> MNNWQHFFNNPVDLSEHLKKPYFRFDNRDKEITAISFDEKANLIWSGDSYGCISSYDPTFQLYTRYRGHIGGNSVKDILSHRDGILSISEDSLHFANRRGVTKLNLTSIDIAAFSELNTMCYSPHSLKNNIYCGGDNTNWGIASIDLNRGCLDSLLNYSSKVKLMCSNNKVLSIGRQTGTVDLLDPTSNRTIKSFNAHSASISAMDLRDNTLVTVGKSKRFYNLYADPFVNVYDLRTMRQLPPVSFSKGTTMGSGGADFVQLHPLLPTVMIVASSSGSFDFIDLSNPTLRTQYVHPCQSIKKLCLSPNGDVLGILEADNHLDTWRRSSNNMGMFTNTPEMLAYPDYFNDITSDGPISVDDETYPLSSVGMPYYLDKLLSAWPPVVFKSEGTIPQLTGKSPLPSSGKLKSNLAVISSQNEKLSTQEFPLLRYDRTKYGMRNAIPDYVCLRDIRKQITSGLETSDIQTYTSINKYEVPPAYSRLPLTSGRFGTDNFDFTPFNNTEYSGLDPDVDNHYTNAIIQLYRFIPEMFNFVVGCLKDENFETTLLTDLGYLFDMMERSHGKICSSSNFQASLKSLTDKRQLENGEPQEHLEEYLESLCIRESIEDFNSSESIKRNMPQKFNRFLLSQLIKEEAQTVNHNITLNQCFGLETEIRTECSCDHYDTTVKLLPSLSISGINKTVIKQLNKKSNGQNILPYIEYAMKNVTQKNSICPTCGKTETITQECTVKNLPSVLSLELSLLDTEFSNIRSSKNWLTSEFYGSIIKNKAVLRSTASELKGTSHIFKYELNGYVAKITDNNNETRLVTYVKKYNPKENCFKWLMFNDYLVVEITEEEALKMTYPWKTPEIIIYCDAEELRKPFFSVDTYSINYDILFRDYFANGIRDTARREYKLLTHDEAPKSGTLVAIDAEFVSLQSELCEIDHQGIRSIIRPKRTALARISIIRGEEGELYGVPFVDDYVVNTNHIEDYLTRYSGILPGDLDPEKSTKRLVRRNVVYRKVWLLMQLGCVFVGHGLNNDFKHININVPRNQIRDTAIYFLQGKRYLSLRYLAYVLLGMNIQEGNHDSIEDAHTALILYKKYLHLKEKAIFEKVLNSVYEEGRAHNFKVPETSKG;>[3x]GPDSMADITDKTAEQLENLNIQDDQKQAATGSESQSVENSSASLYVGDLEPSVSEAHLYDIFSPIGSVSSIRVCRDAITKTSLGYAYVNFNDHEAGRKAIEQLNYTPIKGRLCRIMWSQRDPSLRKKGSGNIFIKNLHPDIDNKALYDTFSVFGDILSSKIATDENGKSKGFGFVHFEEEGAAKEAIDALNGMLLNGQEIYVAPHLSRKERDSQLEETKAHYTNLYVKNINSETTDEQFQELFAKFGPIVSASLEKDADGKLKGFGFVNYEKHEDAVKAVEALNDSELNGEKLYVGRAQKKNERMHVLKKQYEAYRLEKMAKYQGVNLFVKNLDDSVDDEKLEEEFAPYGTITSAKVMRTENGKSKGFGFVCFSTPEEATKAITEKNQQIVAGKPLYVAIAQRKDVRRSQLAQQIQARNQMRYQQATAAAAAAAAGMPGQFMPPMFYGVMPPRGVPFNGPNPQQMNPMGGMPKNGMPPQFRNGPVYGVPPQGGFPRNANDNNQFYQQKQRQALGEQLYKKVSAKTSNEEAAGKITGMILDLPPQEVFPLLESDELFEQHYKEASAAYESFKKEQEQQTEQA;> MHSLLQYHISLYAPEQPSSLKSLLKPNERSADQLFIPNNI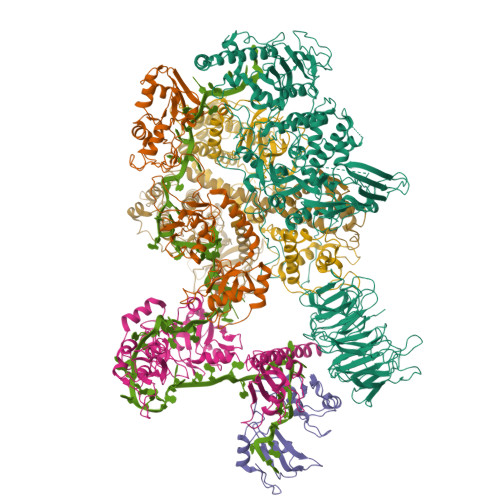REDLTKKNLSILQVFPSSGKVIPSIVQDYFNLVPLNFNNNDFLNKTTLFKVFSNYDGKAYVLKRLPNIDKSMNPNKISKIYQIWSKINCTNLIKFRDIFQTTKFGNLSICLVFDYYPNSLSLYDYHFVNFPKFPITNNYLWIYLVQLTNVINSIHSQNLSIGNTLNWRKVLITGDPGRIKLSHCNFMDLLFNDDTDTVVSSGGSTIEGQQQLDYKYLGELLFNLSINIENSNNNTAPKEYRLEEITPQSIDDMRQIDDKFKDVLKYLISDNGDSKKSIHDLTSHFYDKMFMVLESSQTYTEYMESVLSRELENGRLFRLVNKLNCIFGRIESRIDINWSESGTKFPIILFYDYVFHQVDSNGKPIMDLTHVLRCLNKLDAGIQEKLMLVTPDELNCIIISYKQLKDLIESTFRSITQA;> MDKINPDWAKDIPCRNITIYGYCKKEKEGCPFKHSDNTTATTINDVPPPIDVGEATTPTMTSVPKFNAKVSASFTPMTVGSDSLTTVTNTTSAATNATGNIAMAATSATASTVNPMINPIVNSSLVNNNNNNSNISISIPTTASSSNYDPFNAPIFTPSSTSSIHTNANAHSFPFPSIANSGGININATDDNSNNMSMANNVPPPMQPPPIESSNLKYPRIYPPPHSLLQYHLYAPEQPSSLKSLLKPNERSADQLFIPNNIREDLTKKNLSILQVFPSSGKVIPSIVQDYFNLVPLNFNNNDFLNKTTLFKVFSNYDGKAYVLKRLPNIDKSMNPNKISKIYQIWSKINCTNLIKFRDIFQTTKFGDLSICLVFDYYPNSLSLYDYHFVNFPKFPITNNYLWIYLVQLTNVINSIHSQNLSIGNTLNWRKVLITGDPGRIKLSHCNFMDLLFNDDTDTVVSSGGSTIEGQQQLDYKYLGELLFNLSINIENSNNNTAPKEYRLEEITPQSIDDMRQIDDKFKDVLKYLISDNGDSKKSIHDLTSHFYDKMFMVLESSQTYTEYMESVLSRELENGRLFRLVNKLNCIFGRIESRIDINWSESGTKFPIILFYDYVFHQVDSNGKPIMDLTHVLRCLNKLDAGIQEKLMLVTPDELNCIIISYKELKDLIESTFRSITQHHHHHHHHHH> MMQDATDPAVRAALQSQPSGLNSTDDWRQVMDRIMSLTARNPDAFRQQPQANRLSAILEAVVPARANPTHEKVLAIVNALAENRAIRPDEAGLVYDALLQRVARYNSGNVQTNLDRLVGDVREAVAQRERAQQQGNLGSMVALNAFLSTQPANVPRGQEDYTNFVSALRLMVTETPQSEVYQSGPDYFFQTSRQGLQTVNLSQAFKNLQGLWGVRAPTGDRATVSSLLTPNSRLLLLLIAPFTDSGSVSRDTYLGHLLTLYREAIGQAHVDEHTFQEITSVSRALGQEDTGSLEATLNYLLTNRRQKIPSLHSLNSEEERILRYVQQSVSLNLMRDGVTPSVALDMTARNMEPGMYASNRPFINRLMDYLHRAAAVN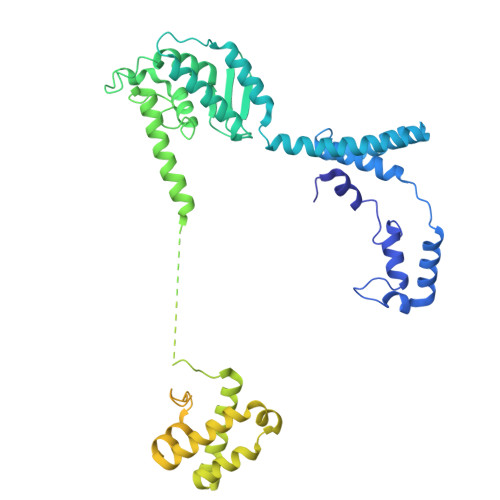PEYFTNAILNPHWLPPPGFYTGGFEVPEGNDGFLWDDIDDSVFSPQPQTLLELQQREQAEAALRKESFRRPSSLSDLGAAAPRSDASSPFPSLIGSLTSTRTTRPRLLGEEEYLNNSLLQPQREKNLPPAFPNNGIESLVDKMSRWKTYAQEHRDVPGPRPPTRRQRHDRQRGLVWEDDDSADDSSVLDLGGSGNPFAHLRPRLGRMF S-[2-({N-[(2R)-2-hydroxy-4-{[(R)-hydroxy(oxo)-lambda~5~-phosphanyl]oxy}-3,3-dimethylbutanoyl]-beta-alanyl}amino)ethyl] 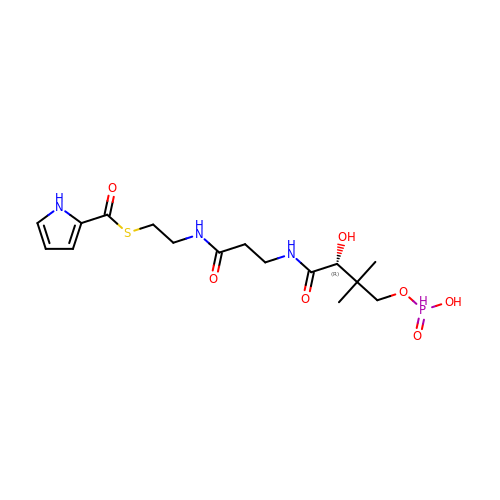1H-pyrrole-2-carbothioate | C16 H26 N3 O7 P S | IYPOXHCBZKSEJQ-ZDUSSCGKSA-N>SNAMGFMIEHWDFSTPMATQETTTAEHIQPNHWYHCERLHPDIRGWLEDNHVPRATVD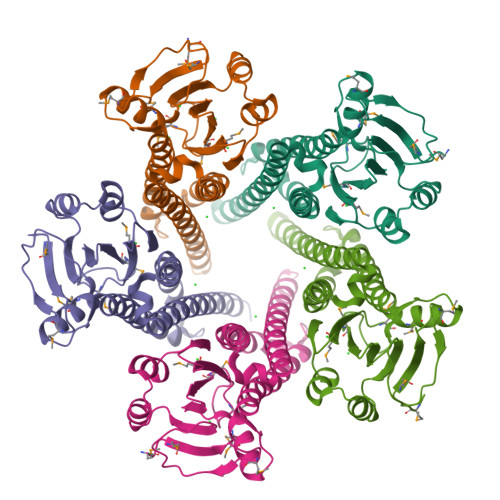HLLADESRPSFHPLDDDNFMLILRGINMNENASPEDMLSIRILYFQGALISTRKIPSRAIMEIRQALAEHKGPKSLASLLNQIIEGLNGKIDLYLDTIEETLNEFDVNDESTYNHIAAQKALISIKRFIRPQQYAIRDLIESESELVTSRPHQYRFAHNNITRINETIEFYLGEVALFQDEIKHNRDEKTNKNS[5x]>RIRIDLPQDEIPAQWYNILPDLPEELPPPQDPTGKSLELLKEVLPSKVLELEFAKERYVKIPDEVLERYLQVGRPTPIIRAKRLEEYLGNNIKIYLKMESYTYTGSHKINSALAHVYYAKLDNAKFVTTETGAGQWGSSVALASALFRMKAHIFMVRTSYYAKPYRKYMMQMYGAEVHPSPSDLTEFGRQLLAKDSNHPGSLGIAISDAVEYAHKNGGKYVVGSVVNSDIMFKTIAGMEAKKQMELIGEDPDYIIGVVGGGSNYAALAYPFLGDELRSGKVRRKYIASGSSEVPKMTKGVYKYDYPDTAKLLPMLKMYTIGSDFVPPPVYAGGLRYHGVAPTLSLLISKGIVQARDYSQEESFKWAKLFSELEGYIPAPETSHALPILAEIAEEAKKSGERKTVLVS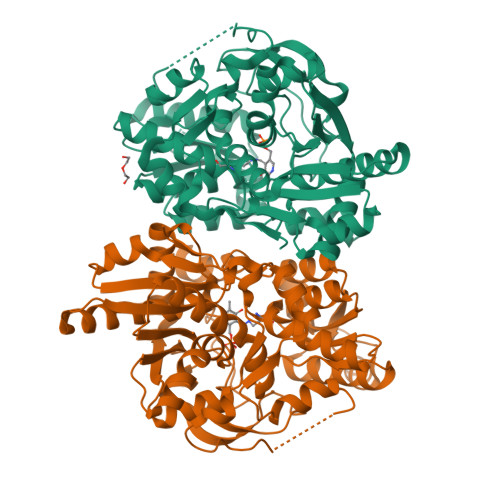FSGHGLLDLGNYASVLFK[2x]6-[3-hydroxy-2-(hydroxymethyl)prop-1-en-1-yl]-4-methoxy-1,5-dimethylpyrimidin-2(1H)-one 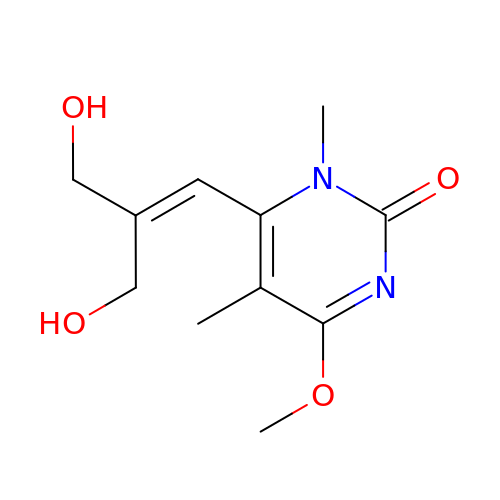| C11 H16 N2 O4 | TVEZWTMUGAPERI-UHFFFAOYSA-N>[4x]MKKLFLVFWWHMHQPLYREPYTGEYLLPWTFFHAVKDYYDMPAYLKDFEIKLNFNLTPVLIDQIQEYAQGKAKDVFLEAIRKDPDDLEKEEVEKLIEFTKLNYEKPIYRFERIRELMNKEKLNREELLDLQTLNLLAWCGRTLRKDLKDLLNKGRNYTQEEKEYVLNKYFE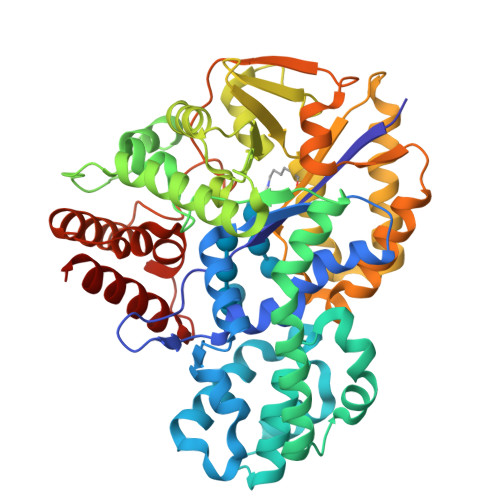IIKKTLSIYREIKEEGKGSVSTSPYYHPLIPILLNPNCVYETTPNVKIPDFAVSFREDASKHVELAKEKYFEIFGEHPVYMWPPQASVSNEALELYYEKGINMLATDEVILKNSVERASPYLRYYFRELISVFFRDKTLSDLIGFSYHAWNAEDAVRDFIGRLKKIHESVDFQPVVFVVLDGENCWEYYEENGIPFLEKLYSTLEKEEWIETLTLEEAMRKEDVKTEVIESVKAGTWFDGNFLKWIGNKEKNEYWKILIEAKKKAKNDYILVAEGSDWFWWQGEEKAPFVEVFDKLFRSFVRRAQE> NTTQQGSPVFAKLLAKNQASLCNTTLNWHSQDGAGSSYLSQGLRYEEDKKELVVDSPGLYYVFLELKLSPTFTNTGHKVQGWVSLVLQAKPQVDDFDNLALTVELFPCSMENKLVDRSWSQLLLLKAGHRLSVGLR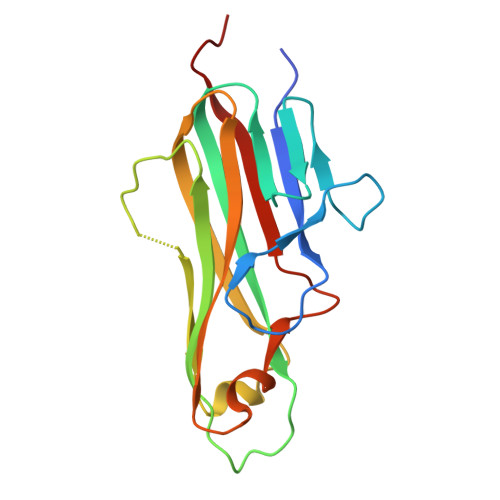AYLHGAQDAYRDWELSYPNTTSFGLFLVKPDNPWE>MKITNPVLKGFNPDPSICRAGEDYYMAVSTFEWFPGVQIYHSKDLIHWRLAARPLQKTSQLDMKGNPDSGGVWAPCLSYADGQFWLIYSDIKVVDGPFKDGHNYLVTADAVDGEWSDPVRLNSSGFDPSLFHDPSGKKYVLNMLWDHREKHHSFAGIALQEYSVS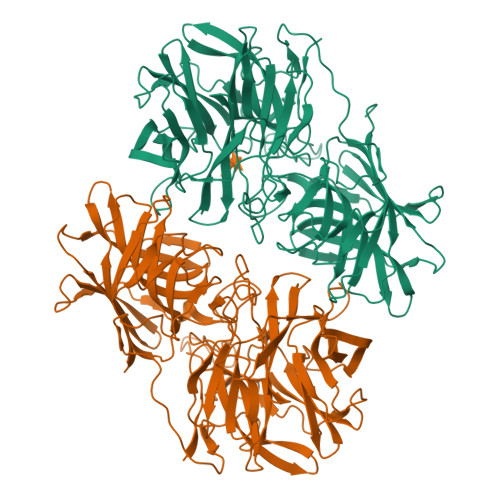EKKLVGERKVIFKGTPIKLTQAPHLYYINDVYYLLTAEGGTRYEHAATIARSSRIDGPYEVHPDNPILTAFHAPSHPLQKCGHASIVQTHTNEWYLAHLTGRPIHSSKESIFQQRGWCPLGRETAIQKLEWKDGWPYVVGGKEGLLEVEAPAMSVKEFSPTYHIVDEFKDSSLNRHFQTLRIPFTDQIGSVTENPHHLRLYGQESLTSKFTQAFVARRWQSFYFEAETAVSFFPKNFQQAAGLVNYYNTENWTALQVTYDDALGRILELSVCENLAFSQPLIKKIIIPDEIPYVYLKVTVQRETYTYSYSFDQQEWEKIDVPLESTHLSDDFIRGGGFFTGAFVGMQCQDTSGERLPADFKYFRYEETTEHHHHHH[4x]8-(1H-imidazol-1-yl)octanoic acid 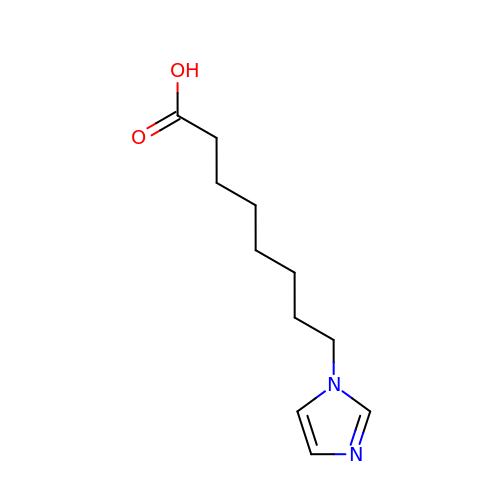| C11 H18 N2 O2 | OUQGDTNNZRAKIB-UHFFFAOYSA-N>MQAVTRFFRHLITLTAVALLAAFLDTVNAAKDTAAGHVTTPCTEILFDLTLAKHYENQIQAAESALNRNYAAIRSWTLLEAMSSDGNRQNAYTGLIAYGIQITVNAEQELQGPKQTKLRAAHALRHRAANLSAALQIQAAQQATLTKPTAGGAQTPFSGATGTCKYEGITATAGEQSCKYSTEDEEKINAAHMNPEVMTQITTIGDKYLTTITLDAIAGSKGNPTQSSATYAEQDCQDGGNPGPNFGGANALGLQVTKLG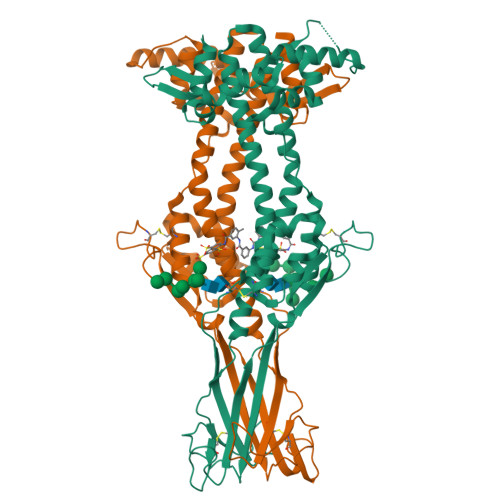TKATTEKTNLYTAGGTECEHQPGNGPQKTKQRLAYLVCEANKAAIITPTDLQTLTLDALISAPEMAAIGDALLTDEPATEKEYSSAQHTQIQQLLKKAYGQTNEQFQKNFIKPLAAQTVKFKIGGAEVSNTVAALMSSPNSGLALAYHKGKNKLQHQVKPDTPLVESKKGSECQVIEDKEKCKTTYGCELKGDKCVVKMTTKGEVTGTQNTTGSNSFVIKKAPLLLAFLLF[2x]4-[1-cyclohexyl-4-(4-fluorophenyl)-1H-imidazol-5-yl]pyrimidin-2-amine | C19 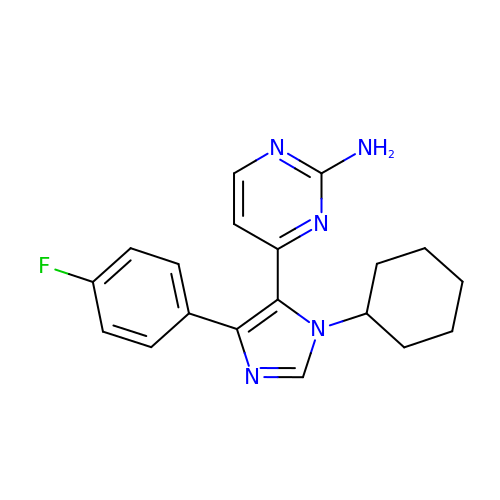H20 F N5 | WUDBUIUHVNECTM-UHFFFAOYSA-N>PPYTVVYFPVRGRCAALRMLLADQGQSWKEEVVTVETWQEGSLKASCLYGQLPKFQDGDLTLYQSNTILRHLGRTLGLYGKDQQEAALVDMVNDGVEDLRCKYISLIYTNYEAGKDDYVKALPGQLKPFETLLSQNQGGKTFIVGDQISFADYNLLDLLL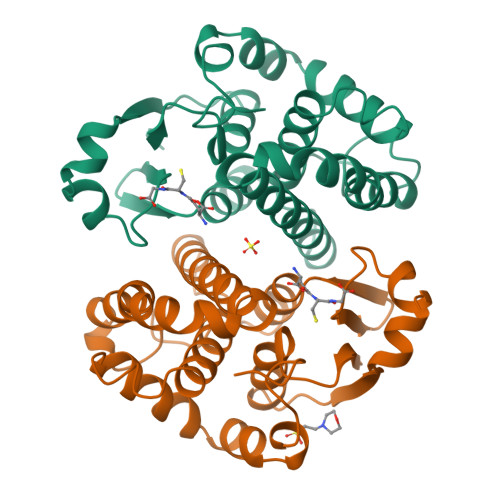IHEVLAPGCLDAFPLLSAYVGRLSARPKLKAFLASPEYVNLPINGNGKQ[3x]>MNMLVINGTPRKHGRTRIAASYIAALYHTDLIDLSE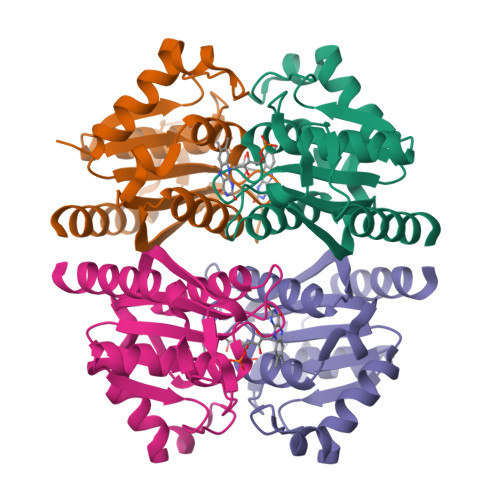FVLPVFNGEAEQSELLKVQELKQRVTKADAIVLLSPEYHSGMSGALKNALDFLSSEQFKYKPVALLAVAGGGDGGINALNNMRTVMRGVYANVIPKQLVLKPVHIDVENATVAENIKESIKELVEELSMFAKAGNPGV[12x]>MFKIGSVLKQIRQELNYHQIDLYSGIMSKSVYIKVEADSRPISVEELSKFSERLGVNFFEILNRAGMNTKSVNETGKEKLLISKIFTNPDLFDKNFQRIEPKRLTSLQYFSIYLGYISIAHHYNIEVPTFNKTITSDLKHLYDKRTTFFGIDYEIVSNLLNVLPYEEVSSIIKP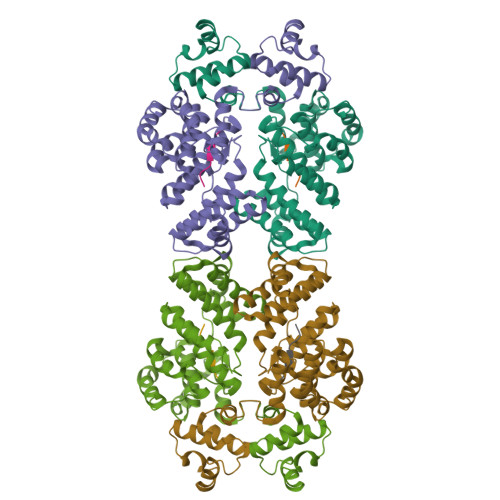MYPIVDSFGKDYDLTIQTVLKNALTISIMNRNLKEAQYYINQFEHLKTIKNISINGCYDLEINYLKQIYQFLTDKNIDSYLNAVNIINIFKIIGKEDIHRSLVEELTKISAKEKFTPPKEVTMYYENYVAIENNPIPEIKEQS[3x];>[2x]AITLIFI>[2x]MSLTGRAFAIPLRTRFRGITVREGMLVRGAAGWGEFSPFAEYGPRECARWWAACYEAAELGWPAPVRDTVPVNATVPAVGPEEAARIVASSGCTTAKVKVAERGQSEANDVARVEAVRDALGPRGRVRIDVNGAWDVDTAVRMIRLLDRFELEYVEQPCATVDELAEVRRRVSVPIAADESIRRAEDPLRVR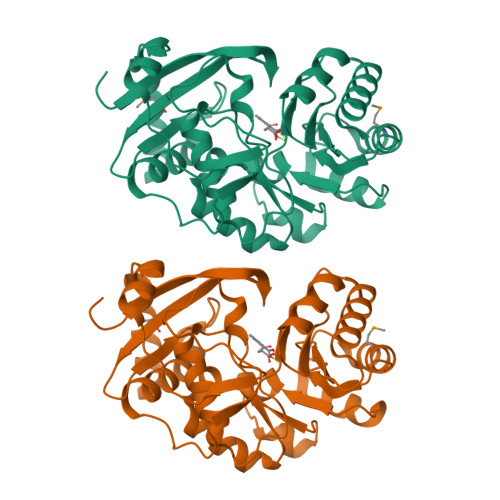DAEAADVVVLKVQPLGGVRAALRLAEECGLPVVVSSAVETSVGLAAGVALAAALPELPYACGLATLRLLHADVCDDPLLPVHGVLPVRRVDVSEQRLAEVEIDPAAWQARLAAARAAWEQVEREPGPEGHHHHHH>GSHMSLIDPRAIIDPSARLAADVQVGPWSIVGAEVEIGEGTVIGPHVVLKGPTKIGKHNRIYQFSSVGEDTPDLKYKGEPTRLVIGDHNVIREGVTIHRGTVQDRAETTIGDHNLIMAYAHIGHDSVIGNHCILVNNTALAGHVHVDDWAILSGYTLVHQYCRIGAHSFSGMGSAIGKDVPAYVTVFGNPAEARSMNFEGMRRRGFS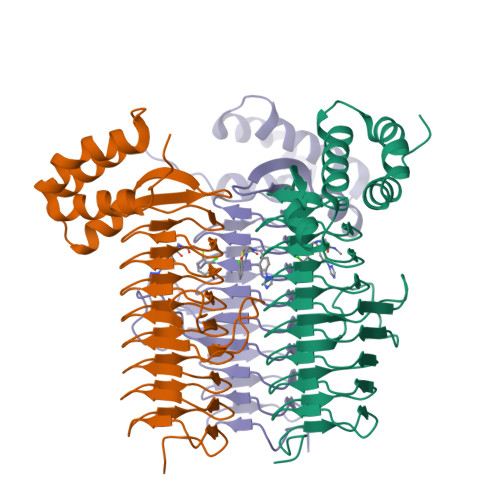SEAIHALRRAYKVVYRQGHTVEEALAELAESAAQFPEVAVFRDSIQSATRGITR[30x]> SSQPNATLYKMSSINADFAFNLYRRFTVETPDKNIFFSPVSISAALVMLSFGACCSTQTEIVETLGFNLTDTPMVEIQHGFQHLICSLNFPKKELELQIGNALFIGKHLKPLAKFLNDVKTLYETEVFSTDFSNISAAKQEINSHVEMQTKGKVVGL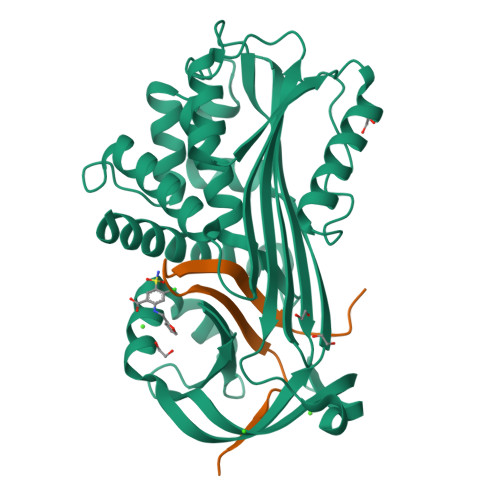IQDLKPNTIMVLVNYIHFKAQWANPFDPSKTEDSSSFLIDKTTTVQVPMMHQMEQYYHLVDMELNCTVLQMDYSKNALALFVLPKEGQMESVEAAMSSKTLKKWNRLLQKGWVDLFVPKFSISATYDLGATLLKMGIQHAYSENADFSGLTEDNGLKLSNAAHKAVLHIGEKGTEAAGAMFLEAIPRSIPNTF;> LHPIIQIDRSFMLLILERSTRSILFLGKVVNPTEA> MSTEQVPVTPDVHYAVEAHYRAEVRLLQTGQYREWLHGMVAEDIHYWMPIY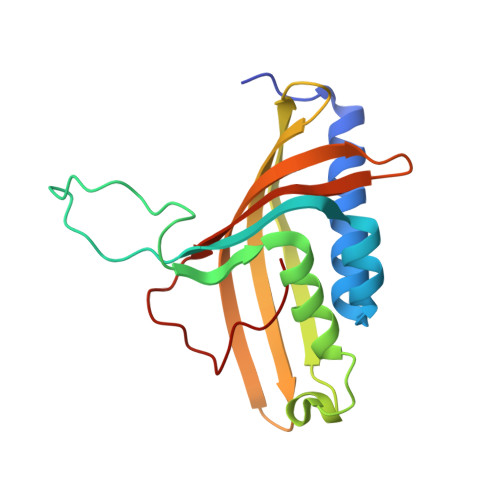EQRFVRDRRPDPTPDDAAIYNDDFEELKQRVERLYSGQVWMEDPPSKIRYFVSNVEAFEAENGELDVLSNILVYRNRRQTEVTVHTLGREDKLRQDGNGFKVFRRKLILDARVTQDKNLYFFC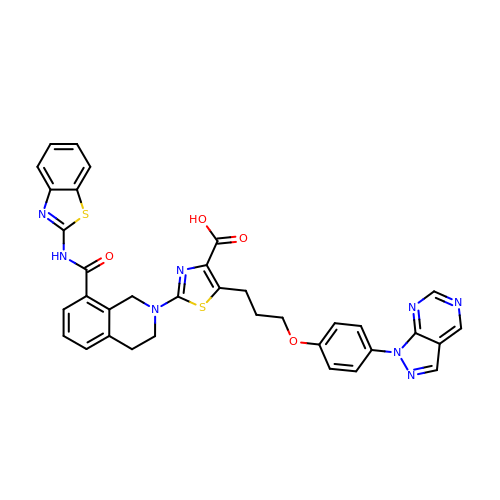2-[8-(1,3-benzothiazol-2-ylcarbamoyl)-3,4-dihydroisoquinolin-2(1H)-yl]-5-{3-[4-(1H-pyrazolo[3,4-d]pyrimidin-1-yl)phenoxy]propyl}-1,3-thiazole-4-carboxylic acid | C35 H28 N8 O4 S2 | LMOJCFKMCAPGGY-UHFFFAOYSA-N>MAANKERTFIMVKPDGVQRGLVGKIIERFEQKGFRLVALKFTWASKELLEKHYADLSARPFFPGLV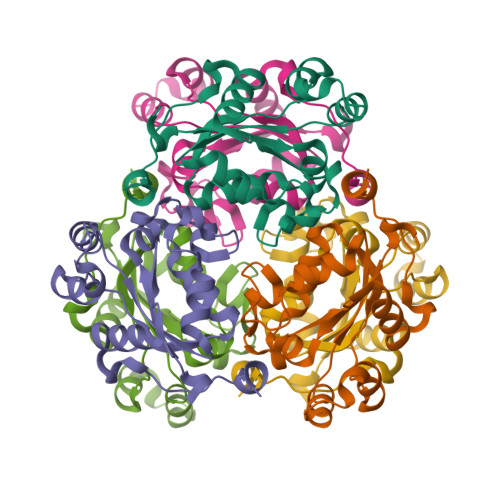NYMNSGPVVPMVWEGLNVVKTGRQMLGATNPADSKPGTIRGDFCIQVGRNIIHGSDAVKSAEKEIALWFNEKELVTWTPAAKDWIYE[3x]>[2x]GPSFWLGNETLKVPLALFALNRQRLCERLRKNPAVQAGSIVVLQGGEETQRYCTDTGVLFRQESFFHWAFGVTEPGCYGVIDVDTGKSTLFVPRLPASHATWMGKIHSKEHFKEKYAVDDVQYVDEIASVLTSQKPSVLLTLRGVNTDSGSVCREASFDGISKFEVNNTILHPEIVECRVFKTDMELEVLRYTNKI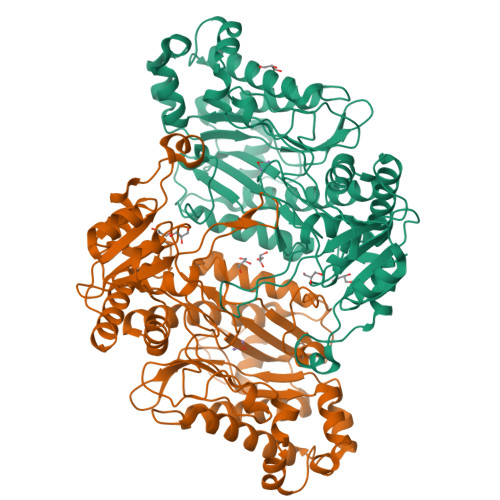SSEAHREVMKAVKVGMKEYELESLFEHYCYSRGGMRHSSYTCICGSGENSAVLHYGHAGAPNDRTIQNGDMCLFDMGGEYYCFASDITCSFPANGKFTADQKAVYEAVLRSSRAVMGAMKPGVWWPDMHRLADRIHLEELAHMGILSGSVDAMVQAHLGAVFMPHGLGHFLGIDVHDVGGYPEGVERIDEPGLRSLRTARHLQPGMVLTVEPGIYFIDHLLDEALADPARASFLNREVLQRFRGFGGVRIEEDVVVTDSGIELLTCVPRTVEEIEACMAGCDKAFTP> MRSLIAMRRRFVSGTWTIAVSTQQRHRSGSGPGDKRIRTDWYRCYPSLMREKDRDMYHCYYPYLFDHGDKMSLYPKIPENPREWQPEQLQTTYDAIREDKYDAFIRLREKFPELYQDTRAWDNPPPFGEFNMFYSVRFGMVGVKAFTCKDYDELGNQFDCTAFWFPDNQVVKHSTRNGEVGTDKVYVGAMNVPVEFHKPHVAAFYKAAGVPVKHVCAGFPITPDAYAPVGTKLDVRHFKPGQEVTITFQNTDYGFRGVMFRHGFDGGYVWLGDSRWQRRPGAMGTEGQKRIYPGHRMAGQTGAAAETYQGVPVWRIDYKNSLIYLPTLLDADVGTYVRFSDTINTKGLTLWNEHRGLPAFPTFIPPEDEDLSKLATDECQLKSPPLYMYFRDEFPATQLVSQ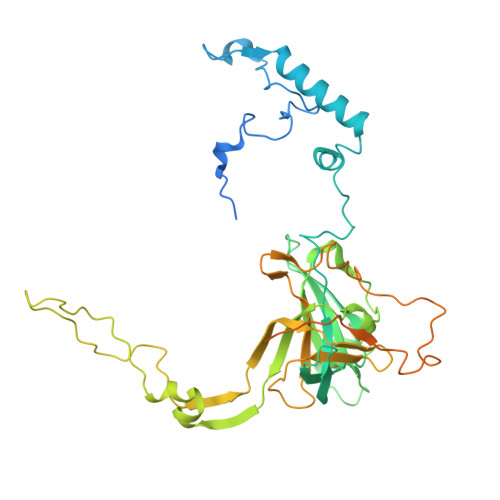ADVEDAKSAKPATAPPKKKVYDMKKYYEARKKYRQSMQKARKYKLMGLRTKAHEKQEEARRAKILKYKRMK> EEVPQDKAPSHVPFLLIGGGTAAFAAARSIRARDPGARVLIVSEDPELPYMRPPLSKELWFSDDPNVTKTLRFKQWNGKERSIYFQPPSFYVSAQDLPHIENGGVAVLTGKKVVQLDVRDNMVKLNDGSQITYEKCLIATGGTPRSLSAIDRAGAEVKSRTTLFRKIGDFRSLEKISREVKSITIIGGGFLGSELACALGRKARALGTEVIQLFPEKGNMGKILPEYLSNWTMEKVRREGVKVM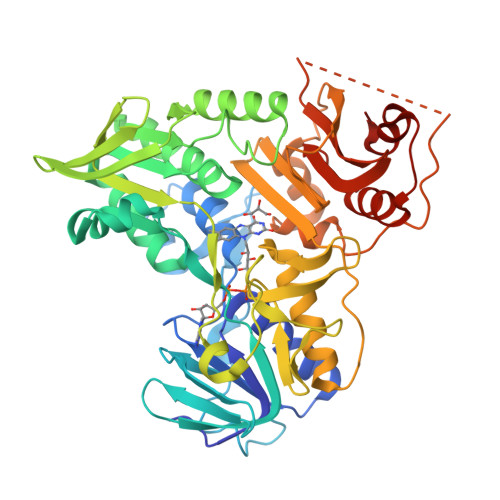PNAIVQSVGVSSGKLLIKLKDGRKVETDHIVAAVGLEPNVELAKTGGLEIDSDFGGFRVNAELQARSNIWVAGDAACFYDIKLGRRRVEHHDHAVVSGRLAGENMTGAAKPYWHQSMFWSDLGPDVGYEAIGLVDSSLPTVGVFAKATAQDNPKSATEQSGTGIRSESETESEASEITIPPSTPAVPQAPVQGEDYGKGVIFYLRDKVVVGIVLWNIFNRMPIARKIIKDGEQHEDLNEVAKLFNIHED>AKVNIKPLEDKILVQANEAETTTASGLVIPDTAKEKPQEGTVVAVGPGRWDEDGEKRIPLDVAEGDTVIYSKYGGTEIKYNGEEYLILSARD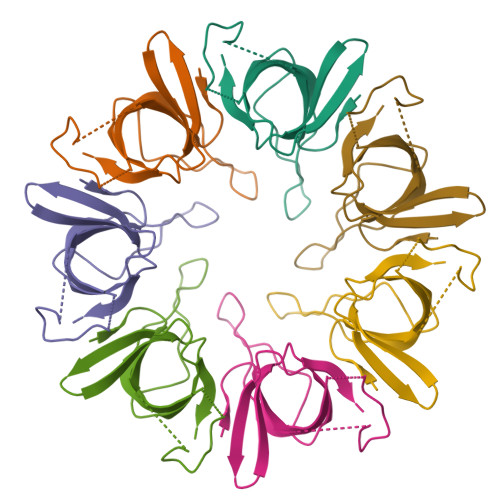VLAVVSK[7x]>CPDACCPHGSSGLRCTRDGALDSLHHLPGAENLTELYIENQQHLQHLELRDLRGLGELRNLTIVKSGLRFVAPDAFHFTPRLSRLNLSFNALESLSWKTVQGLSLQELVLSGNPLHCSCALRWLQRWEEEGLGGVPEQKLQCHGQGPLAHMPNASCGVPTLKVQVPNASVDVGDDVLLRCQVEGRGLEQAGWILTELEQSATVMKSGGLPSLGLTLANVTSDLNRKNVTCWAENDVGRAEVSVQVNVSFPASVQLHTAVEMHHWCIPFSVDGQPAPSLRWLFNGSVLNETSFIFTEFLEPAANETVRHGCLRLNQPTHVNNGNYTLLAANPFGQASASIMAAFMDNP[2x];>SSSHP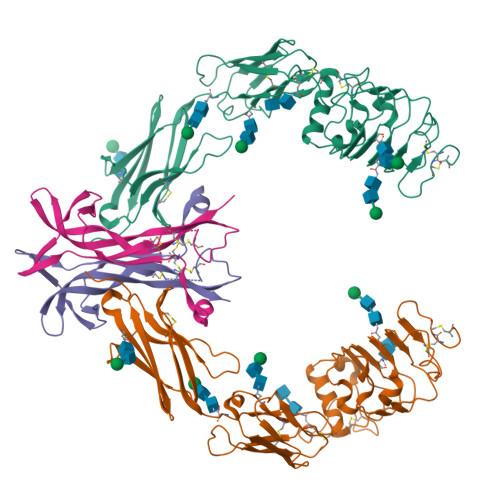IFHRGEFSVCDSVSVWVGDKTTATDIKGKEVMVLGEVNINNSVFKQYFFETKCRDPNPVDSGCRGIDSKHWNSYCTTTHTFVKALTMDGKQAAWRFIRIDTACVCVLSRKAVRRA[2x]>GALQEAVAAQKQEQKTQNQVLQLIAQNWKYFNGNFYYFSRDKKPWREAEKFCTSQGAHLASVTSQEEQAFLVQTTSSGDHWIGLTDQGTEGIW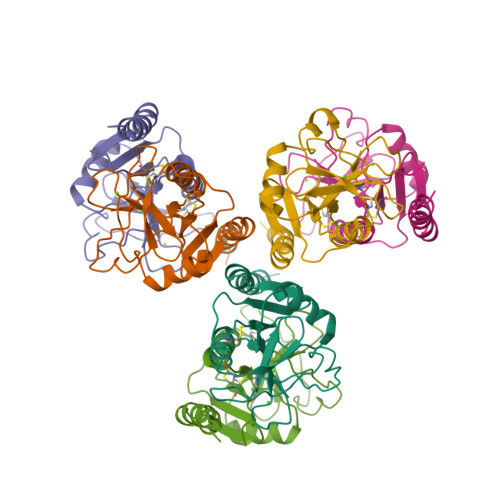RWVDGTPFNNAQSKGFWGKNQPDNWRHRNGEREDCVHVRQQWNDMACGSSYPWVCKKSTGWSAARVG[6x]>MKVVGLDLGGTKIAAGVFDGKRLLSKVVVPTPKEGGERVAEALAEAAERAEREAGVRGEAIGLGTPGPLDFRRGVIRFAPNIPGVQDFPIRRILEEATGRPVFLENDANAAALAEHHLGAAQGEESSLYLTVSTGIGGGVVLGGRVLRGERGQGGELGHLTLLPGGPACGCGLEGCLEALAAGRALERDATYAFQRPVDTRE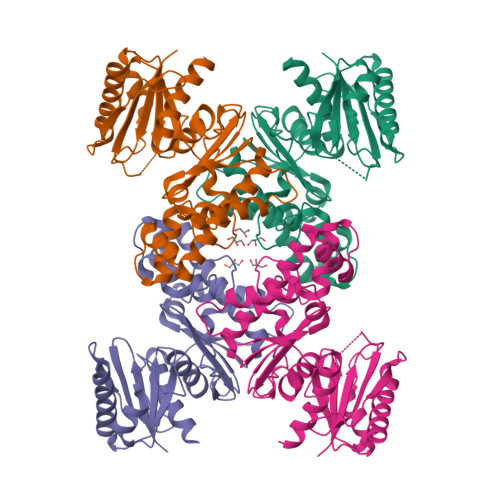LFRLFQAGDPKAERLVLQAARYVGIGLASLVKAFDPGVVVLGGGVALNAPEGYWEALLEAYRRYLQGWEAPPLRRARLGAEAGLLGAALTAYLEVKDGSG[4x]>[2x]EKQPNIDELKKRMEQSRLNKLRGDLDQLIESDPKLRALRPHLKIDLVQEGLRIQIIDSQNRPMFKTG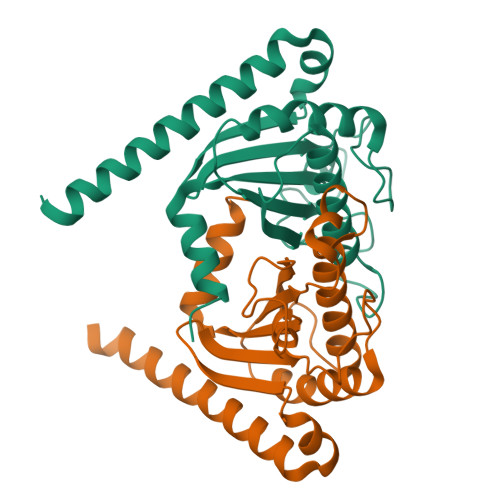SAEVEPYMRDILRAIAPVLNGIPNRISLAGHTDDFPYANGEKGYSNWELSADRANASRRELVAGGLDNGKVLRVVGMAATMRLSDRGPDDAINRRISLLVLNKQAEQAILHHHHHH>[2x]GGA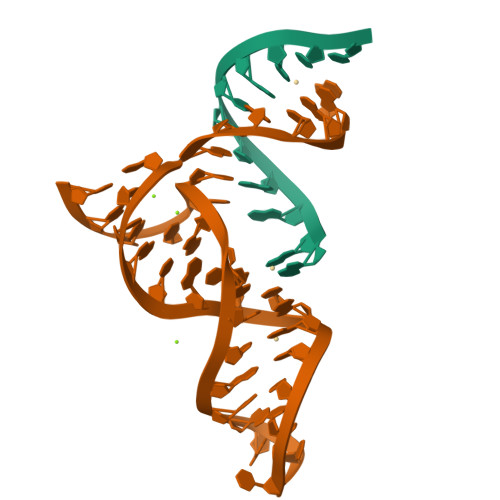GCUCGCCC;>GGGCGAGGCCGUGCCAGCUCUUCGGAGCAAUACUCGGC[2x]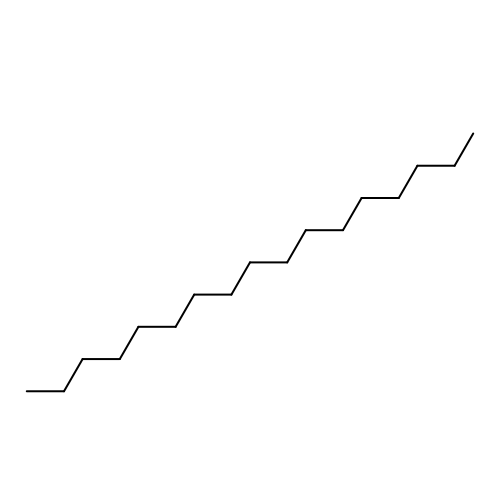heptadecane | C17 H36 | NDJKXXJCMXVBJW-UHFFFAOYSA-N> TSSDTQNNKTLAAMKNFAEQYAKRTDTYFCSDLSVTAVVIEGLARHKEELGSPLCPCRHYEDKEAEVKNTFWNCPCVPMRERKECHCMLFLTPDNDFAGDAQDIPMETLEEVKASMA;> MNVGDRVRVTSSVV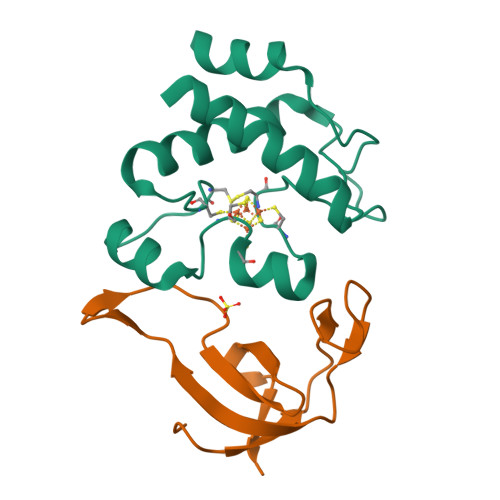VYHHPEHKKTAFDLQGMEGEVAAVLTEWQGRPISANLPVLVKFEQRFKAHFRPDEVTLIED Reverse transcriptases (RTs) use their DNA polymerase and RNase H activities to catalyze the conversion of single-stranded RNA to double-stranded DNA (dsDNA), a crucial process for the replication of retroviruses. Foamy viruses (FVs) have many characteristics that set them apart from OVs, including differences in the proliferation cycle and a different domain structure of the mature RT, which, in addition to POL and RH, harbors the N-terminal protease (PR) domain (PR-RT). Reverse transcriptases have two activities: DNA polymerase (POL) synthesizes DNA on DNA or RNA templates, whereas RNase H (RH) degrades the RNA strand of RNA/DNA hybrid intermediates. The structural and biophysical experiments showed that MFV PR-RT is a monomer upon binding to RNA/DNA and a dimer when it interacts with dsDNA.

The first comprised the full-length PR-RT protein and an RNA/DNA hybrid with 15 bp and overhangs in the RNA strand (a 2-nucleotide [nt] overhang at the 5′ terminus and a 1-nt overhang at the 3′ end [substrate 1]). The sequence of this substrate corresponded to the PPT sequence with the preferred RNase H cut site that was located 13 nt from the recessed 3′ end of the primer. In the structure of full-length PR-RT, the electron density was observed for all four domains: PR, POL, connection, and RNase H. The POL-connection part forms a globular core of the enzyme that is very similar to the p66 subunit of HIV-1 RT and XMRV RT. However, in the present MFV PR-RT structure, the RH domain is well defined because of its stabilization by crystal contacts. In the structure, we observed the electron density for 17 nt of the RNA strand and 15 nt of the DNA strand of the hybrid substrate. It is bound by the POL-connection fragment of MFV PR-RT in a manner that is similar to those of other RTs (HIV-1, XMRV, and Ty3), with the 3′ recessed end of the nucleic acid duplex located at the active site of the POL domain. For the full-length protein, contacts are formed between the POL domain and nt +2 to −6 of the RNA/DNA hybrid. We note, however, that the 3′ end of the DNA in our structure is slightly displaced from the active site, most likely because of the unusual placement of the base of RNA nt +2 in the grove of the hybrid. The fragment of the substrate that comprises nt −8 to −11 interacts with the RH domain of the symmetry-related molecule. Contacts of the RH domain with this part of the substrate result from crystal packing, and such positioning of this domain cannot be accommodated in a single molecule of MFV PR-RT.

> MTTPPLLQLPVEVKKTELNGFWDTGAQITCIPEAFLKEEIPIGEAQIKTLHGTKLQSVYYLKFKVLGRKVEAEVTTSPFDYVIISPSDIPWYKPQPLELTVKLPVQDFKKELINKANINNEEKKQLAKLLDKYDVLWQQWENQVGHRKIPPHNIATGTVAPRPQRQYHINTKAKPSIQQVIDDLLKQGVLIKQTSVMNTPIYPVPKPDGKWRMVLDYRAVNKTVPLIGAQNQHSLGILTNLVRQKYKSTIDLSNGFWAHPITKDSQWITAFTWEGKQHVWTRLPQGFLNSPALFTADVVDLLKNIPGISVYVDDIYFSTETVSEHLKILEKVFKILLEAGYIVSLKKSALLRYEVTFLGFSITQTGRGLTSEFKDKIQNITSPRTLKELQSILGLFNFARNFVPNFSEIIKPLYSLISTAEGNNIKWTSEHTRYLEEIVSALNHAGNLEQRDNESPLVVKLNASPKTGYIRYYNKGGQKPIAYASHVFTNTELKFTPLEKLLVTMHKALIKAIDLALGQPIEVYSPIISMQKLQKTPLPERKALSTRWITWLSYLEDPRITFYYDKTLPDLKNVPETVTDKKPKMLPIIEYAAVFYTNGSAIRSPDKNKSHSSGMGIVHAVFKPELTIEHQWSIPLGDHTAQYAEISAVEFACKKANNISGPVLIVTNSDYVARSVNEELPFWRSNGFVNNKKKPLKHISKWKNISDSLLLKRDIIIVHEPGHKPSYTSIHTQGNNLADKLATQGSYTVNNI> MSEGQIPSSDVLGSQLGVGVQGASLYCPQENYTTKKQEKPQWLRPVDDTLAEDALDLHIVVKSLLCDTAIRYISDDKVLQESDADDDLITSDIDEDTDNQGDTSIVVNPVIPVVPKDVHFFKKVDVGNDSMFGVNCDTPVSFQDYIPSDLLRNLDDTLQESTNSSRPMQDAFFWDPTVANRLDSQYIQTASDLRNYRDGTEIIAYASGKTGSVLNIAVLTRQNTLHLNRHNNVTSIELHSPIKSIKIPGASESIGRRSNLVGIITENSFQIFRIESVHSRSCDVMVSSSEPLYFVEIDDLQVVDFAFNPWDLQQFAIIDIKGNWSIGRIPKNFNNNNKRKLQLIDNLHGTIFDPEELSSWKRIEWFSHFQKILVFDRSKMIEIDFMNNWQTEVVQAKAWSNIRDYKRIDDKNGILLTSREIIIVGASESNDPVRRISWKHDLDPDDTTLRITVQKVKKPDHILLVAFVYSMRHKRIYMHVFSHRKANLFQSLGCSTVLEIPGGTPTGIETILTLDHIDDESRREEDADENFELVVDFLVKLRNSSEVYYYALSNTQNSEPNKQETPIIVDHPEWASLFNNADEREKESIGALVSQIKLKERERISRVQNLIEHENSHDEDKYLQDLGYRLSIATNELLESWQKTKDESILSGSLSHSKLKNLLENSDSFASIPEFSSLLDQFFQYYQDQDVTFIGFEKLLHLFLHEDVPGLDIFYNKLLQCWVLVSPQAELLTKEIVKDIIWSLARLEKPSLFEPIQNEISRSLSGPYQDIISSWDMDDINEEDESNEFNFDSQFSAPFNGRPPFNLNSQSQIPTIKSSQSSGLARRKRILKTQSQKATPLSQSTQNLSVLPDSMTPAFTLMQPPSSQISFVNDSQPRNSQKAKKKK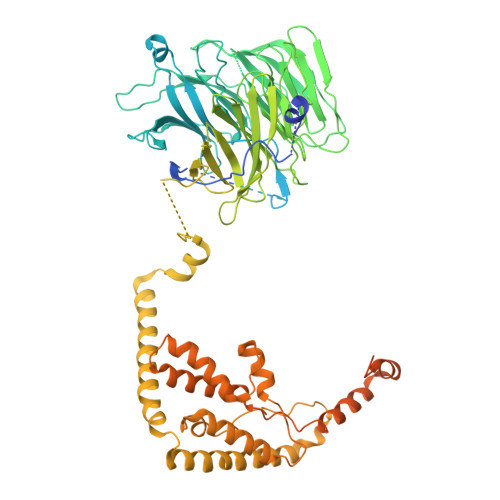KRIRGFG(4R)-2-amino-1,3',3'-trimethyl-7'-(pyrimidin-5-yl)-3',4'-dihydro-2'H-spiro[imidazole-4,1'-naphthalen]-5(1H)-one 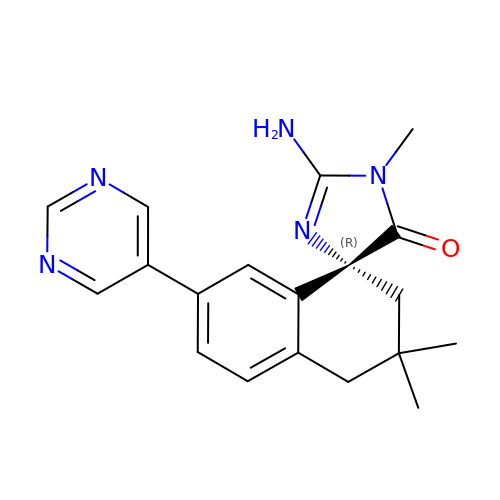| C19 H21 N5 O | UPOMBIAVTOFWMY-LJQANCHMSA-N> MKKSKRKNAQAQEAQETEVLVQEEAEELPEFPEGEPDPDLEDPDLALEDDLLDLPEEGEGLDLEEEEEDLPIPKISTSDPVRQYLHEIGQVPLLTLEEEVELARKVEEGMEAIKKLSEITGLDPDLIREVVRAKILGSARVRHIPGLKETLDPKTVEEIDQKLKSLPKEHKRYLHIAREGEAARQHLIEANLRLVVSIAKKYTGRGLSFLDLIQEGNQGLIRAVEKFEYKRRFKFSTYATWWIRQAINRAIADQARTIRIPVHMVETINKLSRTARQL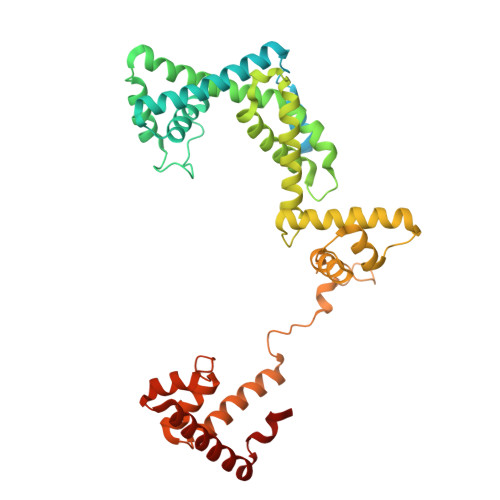QQELGREPTYEEIAEAMGPGWDAKRVEETLKIAQEPVSLETPIGDEKDSFYGDFIPDEHLPSPVDAATQSLLSEELEKALSKLSEREAMVLKLRKGLIDGREHTLEEVGAFFGVTRERIRQIENKALRKLKYHESRTRKLRDFLD>[2x]MVSLVELDPAPIAEDAVVDAPYRIRNYTGFDVIISTKRQIPGASPTTEQQLPTMTLRLEDGQEAPWSFEEWEKMRESLMTESSTANSISVQLVGSGFQEVKSIRLTREGEFLFGLKPKTQQVLHKLLVEIKLGKDNIKYVTLRSPLLVENDTGIVVELGVYDAHEGHLLKIERINPGESKPAPVGAAYFKSLLVRPDPGFKYGWSSDTLWWRDLLKRPTKTLVCKSEQYGGEVFYFRLHARWDQANPLTRNYPYMRLKLTAPLTIENLLPYDFKYKIYDRVNKQEWNNFLRKGGSIPVHMVDLSHTFLLGIEMQDTPFQASEFVVINTGNADDFKKDSHLVVKDNAGMPLNLRLHYFRIPDGGGSFKVTVYSPYVILNKTGLDVSVRSKGFMQSARAAAGQTLIDVGGDGQKKARPLMFSFHNDDHRNRALLKAGDSEWSKPQSFDAIGSTTEVVLQT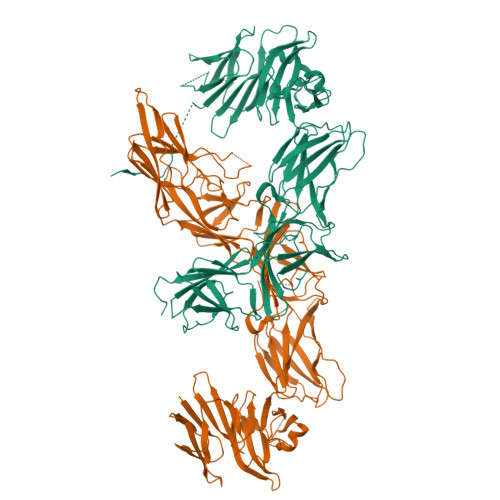ANRNAEIHLGVTVDSGQGKYKMVKVVTLAPRYVIHNKLGEDINIREPSSSFWIPLKHGAHRPLHWLQRGAVKQLCLCYPGVDNQWTAPFNISDLGITHLKIARAGQRQRLIRVEILMEDATIFLNLSMEQRNWPFSMRNESDTEFTFYQVNPTIEEDASEDRSGWRPVRYRLPPRSIMPYAWDFPAAKHKEICICAYNKERHVKLQEIGNLMPMKLALPNGESKTIDINVTADGPTQTLILSNYRQSKSLYRQHHHHHH>[58x]SRSYSQRYAKWQAKFNAFSNPTVASTILSNVSPVAQQNFQTNVPKFTSVNENVSAVL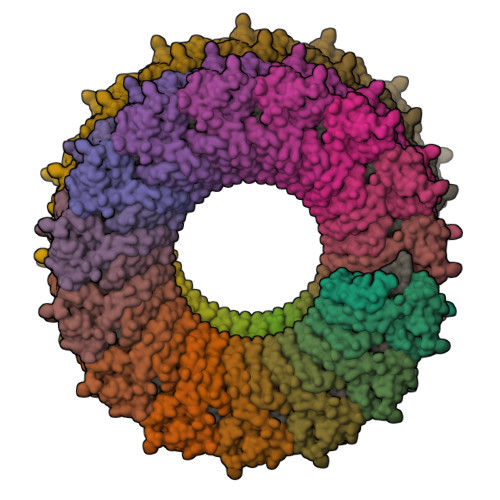TQYGITGPNRAIYQGFGLKVARALNRIGSGPALVNMINGLKGYYISAFNANPQVLDAVVNIITGSPTGYVS> GSGEVTCEPGTTFKDKCNTCRCGSDG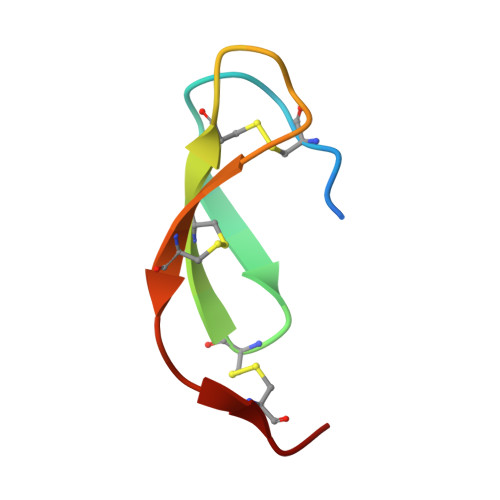KSAVCTKLWCNQ>[76x]MSATASTATQPKPLEWLNRLRANPRIPLIVAGSAAVAIVVAMVLWAKTPDYRTLFSNLSDQDGGAIVAQLTQMNIPYRFANGSGAIEVPADKVHELRLRLAQQGLPKGGAVGFELLDQEKFGISQFSEQVNYQRALEGELARTIETLGPVKSARVHLAMPKPSLFVREQKSPSASVTVTLEPGRALDEGQISAVVHLVSSAVAGLPPGNVTLVDQSGHLLTQSNTSGRDLNDAQLKFANDVESRIQRRIEAILSPIVGNGNVHAQVTAQLDFANKEQTEEHYSPNGDASKATLRSRQLNISEQVGAGYPGGVPGALSNQPAPPNEAPIATPPTNQQNAQNTPQTSTSTNSNSAGPRSTQRNETSNYEVDRTIRHTKMNVGDIERLSVAVVVNYKTLADGKPLPLTADQMKQIEDLTREAMGFSDKRGDTLNVVNSPFSAVDNTGGELPFWQQQSFIDQLLAAGRWLLVLVVAWILWRKAVRPQLTRRVEEAKAAQEQAQVRQETEEAVEVRLSKDEQLQQRRANQRLGAEVMSQRIREMSDNDPRVVALVIRQWMSNDHE;>MTPESVMMMGTEAMKVALALAAPLLLVALITGLIISILQAATQINEMTLSFIPKIVAVFIAIIVAGPWMLNLLLDYVRTLFSNLPYIIG[4x];> MIQVTSEQWLYWLHLYFWPLLRVLALISTAPILSERAIPKRVKLGLGIMITLVIAPSLPANDTPLFSIAALWLAMQQILIGIALGFTMQFAFAAVRTAGEFIGLQMGLSFATFVDPGSHLNMPVLARIMDMLAMLLFLTFNGHLWLISLLVDTFHTLPIGSNPVNSNAFMALARAGGLIFLNGLMLALPVITLLLTLNLALGLLNRMAPQLSIFVIGFPLTLTVGIMLMAALMPLIAPFCEHLFSEIFNLLADIVSEMPINNNP;>[5x]MRRLLFLSLAGLWLFSPAAAAQLPGLISQPLAGGGQSWSLSVQTLVFITSLTFLPAILLMMTSFTRIIIVFGLLRNALGTPSAPPNQVLLGLALFLTFFIMSPVIDKIYVDAYQPFSEQKISMQEALDKGAQPLRAFMLRQTREADLALFARLANSGPLQGPEAVPMRILLPAYVTSELKTAFQIGFTIFIPFLIIDLVIASVLMALGMMMVPPATIALPFKLMLFVLVDGWQLLMGSLAQSFYS;>[6x]MAAIQGIEGVISQLQATAMAARGQDTHSQSTVSFAGQLHAALDRISDRQAAARVQAEKFTLGEPGIALNDVMADMQKASVSMQMGIQVRNKLVAAYQEVMSMQV;>[5x]MLDRLDAALRFQQEALNLRAQRQEILAANIANADTPGYQARDIDFASELKKVMVRGREETGGVALTLTSSHHIPAQAVSSPAVDLLYRVPDQPSLDGNTVDMDRERTQFADNSLKYQMGLTVLGSQLKGMMNVLQGGN;>MALLNIFDIAGSALAAQSKRLNVAASNLANADSVTGPDGQPYRAKQVVFQVDAAPGQATGGVKVASVIESQAPEKLVYEPGNPLADANGYVKMPNVDVVGEMVNTMSASRSYQANIEVLNTVKSMMLKTLTLGQ[6x]

The bacterial flagellar motor is a huge bidirectional rotary nanomachine that drives rotation of the flagellum for bacterial motility. The cytoplasmic C ring of the flagellar motor functions as the switch complex for the rotational direction switching from counterclockwise to clockwise. The basal body is made up of the LP ring, MS ring, C ring, rod and export apparatus. Here, we present two high-resolution cryo-electron microscopy structures of the C ring-containing flagellar basal body–hook complex from Salmonella Typhimurium, which are in the default counterclockwise state and in a constitutively active CheY mutant-induced clockwise state, respectively.

To obtain the C ring-containing basal body–hook complex in the CW state, we constructed the constitutively active double mutant D13K/Y106W of CheY (hereafter referred to as CheY**), which can mimic CheY-P to tightly bind to the C ring and lock the rotational direction of the motor in the CW state. The density maps of the LP ring, MS ring, rod, hook, and export apparatus in the CW state were locally reconstructed to the higher resolutions ranging from 2.8 Å to 3.8 Å. The MS ring is located on the inner membrane, houses the export apparatus and forms the assembly base for the C ring. In the intact C ring-containing basal body–hook complexes, the MS ring is more stable and harbors much more clear densities for the outer RBM1 subring, outer RBM2 subring and putative inner RBM1 subring, which are made up of 11 RBM1, 11 RBM2 and 23 RBM1 domains of FliF, respectively. In the intact C ring-containing basal body–hook complexes, there is one more peptide loop L3, which consists of the residues G310–P322 of FliF and is also extended from the β-collar region of the MS ring, bound in a hydrophobic groove that is formed by the α2–α3 linking loop of FliE6 with the D0 and DC domains of FlgC1 and FlgC6 on the surface of the rod. The interaction manner of L3 with the rod is different from those of L1 and L2 loops with the rod in the structure of the C ring-free flagellar motor. Thus, there are totally 11 FliF loops that extend from the MS ring to bind the rod in the basal body for torque transmission. These 11 loops are possibly derived from the FliF subunits in the 11-fold outer RBM1–RBM2 subrings. The more stable MS ring in the C ring-containing basal body–hook complexes indicates that the C ring is also important for the stability of the MS ring during motor assembly. Although the structures of the LP ring, MS ring, rod, hook, and export apparatus in the CW state are highly similar to those of these components in the CCW state, the protomers of the C ring in the CW state notably undergo inclination and compaction, suggesting that the binding of CheY** induces significant conformational changes of the C ring for rotational switching.>XP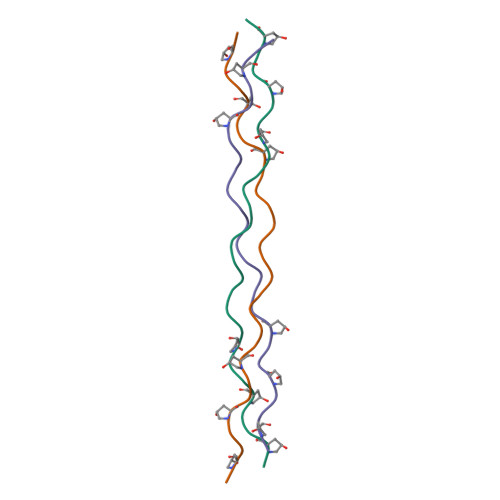PGPPGPPGQRGERGFPGPPGPPGPPG[3x]> GMRKHPQTATKHLFVSGGVASSLGKGLTASSLGQLLTARGLHVTMQKLDPYLNVDPGTMNPFQHGEVFVTEDGAETDLDVGHYERFLDRNLPGSANVTTGQVYSTVIAKERRGEYLGDTVQVIPHITDEIKRRILAMAQPDADGNRPDVVITEIGGTVGDIESQPFLEAARQVRHYLGREDVFFLHVSLVPYLAPSGELKTKPTQHSVAALRSIGITPDALILRCDRDVPEALKNKIALMCDVDIDGVISTPDAPSIYDIPKVLHREELDAFVVRRLNLPFRDVDWTEWDDLLRRVHEPHETVRIALVGKYVELSDAYLSVAEALRAGGFKHRAKVEICWVASDGCETTSGAAAALGDVHGVLIPGGFGIRGIEGK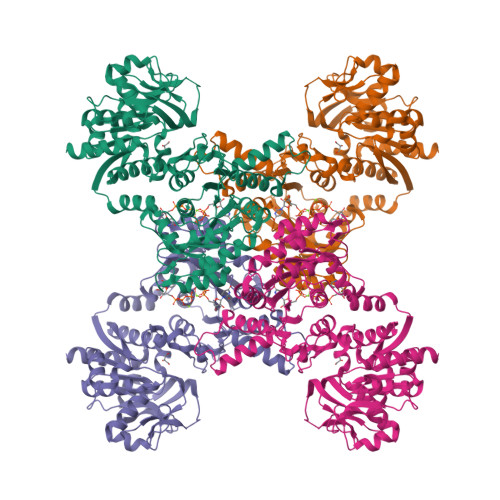IGAIAYARARGLPVLGLCLGLQCIVIEAARSVGLTNANSAEFDPDTPDPVIATMPDQEEIVAGEADLGGTMRLGSYPAVLEPDSVVAQAYQTTQVSERHRHRYEVNNAYRDKIAESGLRFSGTSPDGHLVEFVEYPPDRHPFVVGTQAHPELKSRPTRPHPLFVAFVGAAIDYKAGELLPVEIPEIPEHTPNGSSHRDGVGQPLPEPASRG>QIRYPVPEESQEGTFVGNVAQDFLLDTESLSARRLQVAGEVNQRHFRVDLDSGALLIKNPIDREALCGLSASCIVPLEFVTEGPLEMYRAEVEIVDVNDHAPRFPRQQLDLEIGEAAPPGQRFPLEKAQDADVGSNSISSYRLSSNEHFALDVKKRSDGSLVPELLLEKPLDREKQSDYRLVLTAVDGGNPPRSGTAELRVSVLDVNDNAPAFQQSSYRISVLESAPAGMVLIQLNASDPDLGPSGNVTFSFSGHTPDRVRNLFSLHPTTGKLTLQGPLDFESENYYEFDVRARDGGSPAMEQHCSLRVDL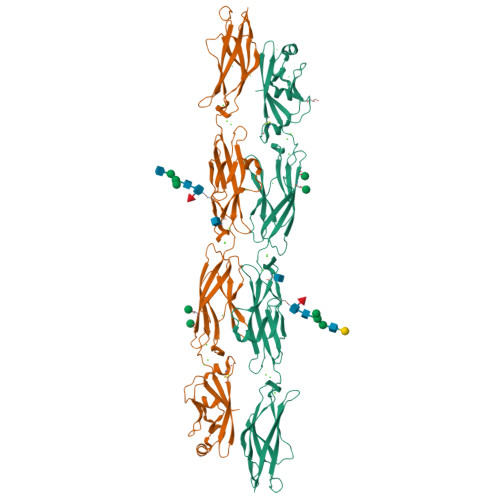LDVNDNAPHITVTSELGTLPESAEPGTVVALISVQDPDSGSNGDVSLRIPDHLPFALKSAFRNQFSLVTAGPLDREARSSYDIMVTASDAGNPPLSTHRTIFLNISDVNDHHHHHHHH[2x]>[4x]GSHMVGDNKLDDKNIDKEKESSYRFPVIAMKVKKGILSDYLSLNGDVDTKVKADIFPDAVGKITSLRIKLGAYVQKGQIVATLDPSRPGSVYLKSPVRAPISGYILNITKKIGETVNPQSNIAVVGRIDTKQILTYVSEKY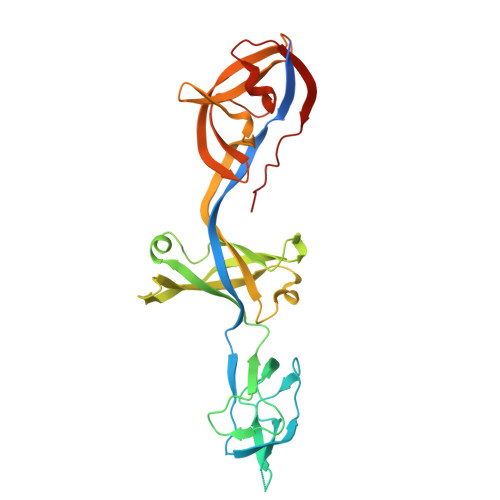ISNIKVGNDAIIEVGAYSNEKFKAKVSEISPILDSKSRTIEVYLTPIGSNLDKLIIGMFSKIKLITKRFKDVIKISREAVVEREGKKFVFKVDLESKSVQMLPITVLFEIDNIVALSGEVEENDLIVVEGMSALSNGSLINLVDTKEGLSAESNI Here, inspired by natural and re-engineered protein–peptide systems, we set out to design proteins made out of repeating units that bind peptides with repeating sequences, with a one-to-one correspondence between the repeat units of the protein and those of the peptide. We use geometric hashing to identify protein backbones and peptide-docking arrangements that are compatible with bidentate hydrogen bonds between the side chains of the protein and the peptide backbone. We design repeat proteins to bind to six different tripeptide-repeat sequences in polyproline II conformations. The proteins are hyperstable and bind to four to six tandem repeats of their tripeptide targets with nanomolar to picomolar affinities in vitro and in living cells.

Reasoning that proline-containing peptides would incur a lower entropic cost upon binding than non-proline-containing peptides, we decided to start our experimental characterization with designs containing at least one proline residue; in most of these designs, the peptide backbone is in or near the polyproline II portion of the Ramachandran map. For the polyproline helix, there are roughly three residues per turn, and, probably because of this, we obtained more designs that target three-residue than two-residue proline-containing repeat units. Crystal structures reveal repeating interactions between protein and peptide interactions as designed, including ladders of hydrogen bonds from protein side chains to peptide backbones. Our results show that by matching superhelical parameters between repeating-protein and repeating-peptide conformations, and incorporating specific hydrogen-bonding and hydrophobic interactions between matched protein and peptide repeats, we can now design modular proteins that bind to extended peptides with high affinity and specificity.

> PEEERIKYVITVVEQIAKDAHRNGQEELAKLAERTAEEAKKATERGEEETLRIVYVIVVVLQIALEAHRNGQEELAKLALRTAEEAIKATERGEEETLRIVYVIVVVLQIALEAHRNGQEELAKLALRTAEEAIKATERGEEETLRIVYVIVVVLQIALEAHRNGQEELAKLALRTAEEAIKATERGEEETLRIVYVIVVVLQIALEAHRNGQEELAKLALRTAEEAIKATERGEEETERIVYDIVVVLQEALEAHRNGEEERAKKALDEARRRIEATERGE;>PLPPLPPLPPLPPLPPLPPLP[2x]N4-like phages have a genome size of about 75 kb, nearly twice that of T7, and encode around 70–90 ORFs, including a characteristic large virion-associated RNA polymerase (vRNAP) unique to this family of bacterial viruses. The massive 3,500-residue vRNAP 18,19, present in 4 ± 1 copies inside the mature virion 20, is ejected into the host upon infection. In stark contrast to the N4 transcriptional program, which has been studied extensively 17, many key questions about the role of phage N4 vRNAP as an ejection protein and its part in the DNA ejectosome remain unanswered. vRNAP (gp50) consists of three predicted domains: a likely membrane-spanning N-terminal domain (NTD), a single-subunit RNA polymerase (RNAP) domain, and a large C-terminal domain of unknown function (CTD). In this study, we use a complementary top-down and bottom-up approach by determining the cryo-EM structures of both the full-length recombinantly expressed vRNAP and the fully asymmetric N4 virion tail.

Single particle analysis (SPA) of cryomicrographs revealed a heterogeneous mix of particles with two predominant and two minor populations. 1007–2101) and a tightly bound complex of RNAP and CTD with an unresolved NTD, referred to as ΔNv-RNAP tight complex (res. N4 isolated RNAP and ΔN-vRNAP tight complex were real-space refined to a model to map correlation coefficients of CC = 0.90 and 0.84, respectively. The tight complex of the RNAP and CTD forms a compact structure where the CTD binds the RNAP on the opposing face of the DNA hairpin promoter binding site 24, leaving the region open for promoter binding. Despite a large binding interface of 1,659 Å2, PISA analysis of the C2 and RNAP interface indicates a weak interaction with a ΔG of nearly zero at −0.2. Interestingly, interactions are slightly stronger at a ΔG of Ȓ2.1 for RNAP to C1 with a 725 Å2 interface. A salt bridge between D2012 (RNAP) and R2279 (C1) likely serves as a clasp for stabilizing the tight complex, which is not predicted to be stable in solution. The CTD buries a large surface area of the RNAP occupied by the fingers and palm including the palm insertion and extended foot domains, but despite the extensive interface, the overall structure of the N4 RNAP domain is relatively unchanged in complex with the CTD (RMSD 3.7 Å), barring a few changes in subdomains unique to N4 and a subtle shift of the fingers. Cryo-EM reconstructions of the four high-resolution states provide clear evidence that the CTD drives the B-motif loop into the active site in a conformation that we predict is inactive. Although the CTD makes sparse contacts with RNAP, it allosterically regulates three crucial motifs of the RNAP core: the intercalating beta-hairpin, the B-motif loop, and the N4 plug module, thereby repressing transcriptional activity.

> MSVFDRLAGFADSVTNAKQVDVSTATAQKKAEQGVTTPLVSPDAAYQMQAARTGNVGANAFEPGTVQSDFMNLTPMQIMNKYGVEQGLQLINARADAGNQVFNDSVTTRTPGEELGDIATGVGLGFVNTLGGIGALGAGLLNDDAGAVVAQQLSKFNDAVHATQSQALQDKRKLFAARNLMNEVESERQYQTDKKEGTNDIVASLSKFGRDFVGSIENAAQTDSIISDGLAEGVGSLLGAGPVLRGASLLGKAVVPANTLRSAALAGAIDAGTGTQSLARIASTVGRAAPGMVGVGAMEAGGAYQQTADEIMKMSLKDLEKSPVYQQHIKDGMSPEQARRQTASETGLTAAAIQLPIAAATGPLVSRFEMAPFRAGSLGAVGMNLARETVEEGVQGATGQLAQNIAQQQNIDKNQDLLKGVGTQAGLGALYGFGSAGVVQAPAGAARLAGAATAPVLRTTMAGVKAAGSVAGKVVSPIKNTLVARGERVMKQNEEASPVADDYVAQAAQEAMAQAPEAEVTIRDAVEATDATPEQKVAAHQYVSDLMNATRFNPENYQEAPEHIRNAVAGSTDQVQVIQKLADLVNTLDESNPQALMEAASYMYDAVSEFEQFINRDPAALDSIPKDSPAIELLNRYTNLTANIQNTPKVIGALNVINRMINESAQNGSLNVTEESSPQEMQNVALAAEVAPEKLNPESVNVVLKHAADGRIKLNNRQIAALQNAAAILKGAREYDAEAARLGLRPQDIVSKQIKTDESRTQEGQYSALQHANRIRSAYNSGNFELASAYLNDFMQFAQHMQNKVGALNEHLVTGNADKNKSVHYQALTADREWVRSRTGLGVNPYDTKSVKFAQQVALEAKTVADIANALASAYPELKVSHIKVTPLDSRLNAPAAEVVKAFRQGNRDVASSQPKADSVNQVKETPVTKQEPVTSTVQTKTPVSESVKTEPTTKESSPQAIKEPVNQSEKQDVNLTNEDNIKQPTESVKETETSTKESTVTEELKEGIDAVYPSLVGTADSKAEGIKNYFKLSFTLPEEQKSRTVGSEAPLKDVAQALSSRARYELFTEKETANPAFNGEVIKRYKELMEHGEGIADILRSRLAKFLNTKDVGKRFAQGTEANRWVGGKLLNIVEQDGDTFKYNEQLLQTAVLAGLQWRLTATSNTAIKDAKDVAAITGIDQALLPEGLVEQFDTGMTLTEAVSSLAQKIESYWGLSRNPNAPLGYTKGIPTAMAAEILAAFVESTDVVENIVDMSEIDPDNKKTIGLYTITELDSFDPINSFPTAIEEAVLVNPTEKMFFGDDIPPVANTQLRNPAVRNTPEQKAALKAEQATEFYVHTPMVQFYETLGKDRILELMGAGTLNKELLNDNHAKSLEGKNRSVEDSYNQLFSVIEQVRAQSEDISTVPIHYAYNMTRVGRMQMLGKYNPQSAKLVREAILPTKATLDLSNQNNEDFSAFQLGLAQALDIKVHTMTREVMSDELTKLLEGNLKPAIDMMVEFNTTGSLPENAVDVLNTALGDRKSFVALMALMEYSRYLVAEDKSAFVTPLYVEADGVTNGPINAMMLMTGGLFTPDWIRNIAKGGLFIGSPNKTMNEHRSTADNNDLYQASTNALMESLGKLRSNYASNMPIQSQIDSLLSLMDLFLPDINLGENGALELKRGIAKNPLTITIYGSGARGIAGKLVSSVTDAIYERMSDVLKARAKDPNISAAMAMFGKQAASEAHAEELLARFLKDMETLTSTVPVKRKGVLELQSTGTGAKGKINPKTYTIKGEQLKALQENMLHFFVEPLRNGITQTVGESLVYSTEQLQKATQIQSVVLEDMFKQRVQEKLAEKAKDPTWKKGDFLTQKELNDIQASLNNLAPMIETGSQTFYIAGSENAEVANQVLATNLDDRMRVPMSIYAPAQAGVAGIPFMTIGTGDGMMMQTLSTMKGAPKNTLKIFDGMNIGLNDITDASRKANEAVYTSWQGNPIKNVYESYAKFMKNVDFSKLSPEALEAIGKSALEYDQRENATVDDIANAASLIERNLRNIALGVDIRHKVLDKVNLSIDQMAAVGAPYQNNGKIDLSNMTPEQQADELNKLFREELEARKQKVAKARAEVKEETVSEKEPVNPDFGMVGREHKASGVRILSATAIRNLAKISNLPSTQAATLAEIQKSLAAKDYKIIYGTPTQVAEYARQKNVTELTSQEMEEAQAGNIYGWTNFDDKTIYLVSPSMETLIHELVHASTFEEVYSFYQGNEVSPTSKQAIENLEGLMEQFRSLDISKDSPEMREAYADAIATIEGHLSNGFVDPAISKAAALNEFMAWGLANRALAAKQKRTSSLVQMVKDVYQAIKKLIWGRKQAPALGEDMFSNLLFNSAILMRSQPTTQAVAKDGTLFHSKAYGNNERLSQLNQTFDKLVTDYLRTDPVTEVERRGNVANALMSATRLVRDVQSHGFNMTAQEQSVFQMVTAALATEAAIDPHAMARAQELYTHVMKHLTVEHFMADPDSTNPADRYYAQQKYDTISGANLVEVDAKGRTSLLPTFLGLAMVNEELRSIIKEMPVPKADKKLGNDIDTLLTNAGTQVMESLNRRMAGDQKATNVQDSIDALSETIMAAALKRESFYDAVATPTGNFIDRANQYVTDSIERLSETVIEKADKVIANPSNIAAKGVAHLAKLTAAIASEKQGEIVAQGVMTAMNQGKVWQPFHDLVNDIVGRTKTNANVYDLIKLVKSQISQDRQQFREHLPTVIAGKFSRKLTDTEWSAMHTGLGKTDLAVLRETMSMAEIRDLLSSSKKVKDEISTLEKEIQNQAGRNWNLVQKKSKQLAQYMIMGEVGNNLLRNAHAISRLLGERITNGPVADVAAIDKLITLYSLELMNKSDRDLLSELAQSEVEGMEFSIAYMVGQRTEEMRKAKGDNRTLLNHFKGYIPVENQQGVNLIIADDKEFAKLNSQSFTRIGTYQGSTGFRTGSKGYYFSPVAARAPYSQGILQNVRNTAGGVDIGTGFTLGTMVAGRITDKPTVERITKALAKGERGREPLMPIYNSKGQVVAYEQSVDPNMLKHLNQDNHFAKMVGVWRGRQVEEAKAQRFNDILIEQLHAMYEKDIKDSSANKSQYVNLLGKIDDPVLADAINLMNIETRHKAEELFGKDELWVRRDMLNDALGYRAASIGDVWTGNSRWSPSTLDTVKKMFLGAFGNKAYHVVMNAENTIQNLVKDAKTVIVVKAVVVPAVNFLANIYQMIGRGVPVKDIAVNIPRKTSEINQYIKSRLRQIDAEAELRAAEGNPNLVRKLKTEIQSITDSHRRMSIWPLIEAGEFSSIADAGISRDDLLVAEGKIHEYMEKLANKLPEKVRNAGRYALIAKDTALFQGIQKTVEYSDFIAKAIIYDDLVKRKKKSSSEALGQVTEEFINYDRLPGRFRGYMESMGLMWFYNFKIRSIKVAMSMIRNNPVHSLIATVVPAPTMFGNVGLPIQDNMLTMLAEGRLDYSLGFGQGLRAPTLNPWFNLTH>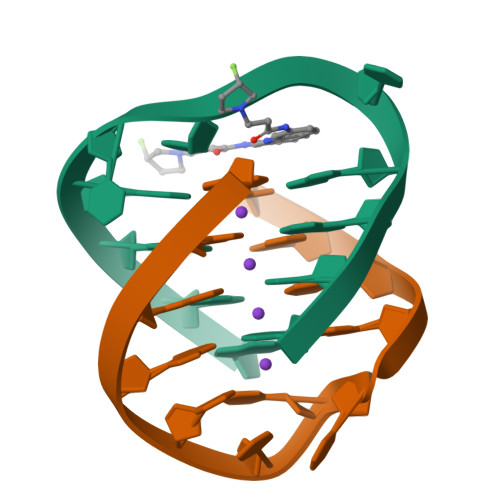[2x]GGGGTTTTGGGG>[4x]MVKKPSLAGRLKIIEIDGRKTLGDQHGNPIQLRGMSTHGLQWFPQIINNNAFSALSKDWEANVIRLAMYVGEGGYSTDPSVKEKVIEGINLAIKNDMYVIVDWHILNPGDPNAKIYSGAKEFFKEIASKYPNDLHIIYELANEPNPTESDITNDIAGWEKVKKYAEPIIKMLRDMGNENIIIVGNPEWSTRPDLAVNDPIDDKNVMYSAHFYTGSASVWENGNKGHIARNIEKALENGLTVFVTEWGTSEASGDGGPYLNEADEWLEFLNSNNISWVNWSLANKNEASAAFLPTTSLDPGNGKVWAVNQLSLSGEYVRARIKGIPYKPISRETM

In this study, a new thermotolerant and exceptionally halostable GH5 cellulase from an Icelandic Thermoanaerobacterium hot spring isolate was identified and characterized. Thus, we conclude that CelDZ1 is a novel endo-glucanase for soluble cellulose. CelDZ1 has an (β/α)8-barrel structure with two additional β-hairpins, one at its N terminus and another preceding helix α6. All of the catalytic residues are conserved with Glu192 and Glu294 found on the C termini of the barrel strands β4 and β7, which are the acid/base and the nucleophile for catalysis, respectively.

The CelDZ1α structure has been determined and refined to an R-cryst/R-free of 19.3/23.4% for all data to 1.9 Å without σ cutoff. The N-terminal 49 amino acids forming the transmembrane helix and a linker to the catalytic domain were not defined due to disorder in the crystal. Out of the four monomers that make up the asymmetric unit of the enzymes crystal only two monomers, A and B, were clearly defined in the electron density since they are more restricted by many crystal contacts. The other two monomers, C and D, form fewer crystal contacts and are less well ordered. The CelDZ1 model also contained 585 ordered water molecules and several ordered isopropanol, ethylene glycol and polyethylene glycol molecules that were present in the crystal cryoprotectant. Although the asymmetric unit of CelDZ1 crystal contains four monomers, these do not form oligomers in the crystal according to PISA. The residues Pro157, Pro306 and Ser329 are in the cis conformation in CelDZ1. Whilst both the CelK and Cel5A enzymes have the distinct 2 subsite, where the residues Gln180 and His206 (Cel5A numbering) form H-bonds to the oxygens of the glucose unit at this position, neither of these residues are conserved in CelDZ1 where Thr239/Ala265 replaces the equivalent Gln/His residues. The two residues of CelDZ1 are unable to form a sugar-binding subsite and there are no apparent nearby residues capable of binding a sugar unit. CelDZ1 thus appears to be the first cellulose structure lacking the sugar-binding 2 subsite.>[6x]MLAFPKEFWWGGATSGPQSEGRFAKQHRNLFDYWYEEEPDLFYDYVGPDTASDAYHQIESDLTLLASLGHNSYRTSIQWTRLIDDFEQATINPDGLAYYNRVIDACLANGIRPVINLHHFDLPIALYQAYGGWESKHVVDLFVAFSKVCFEQFGDRVKDWFVHNEPMVVVEGSYLMQFHYPAIVDGKKAVQVAYNLALATAKVIQAYRRGPAELSDGRIGTILNLTPAYPASQSEADMA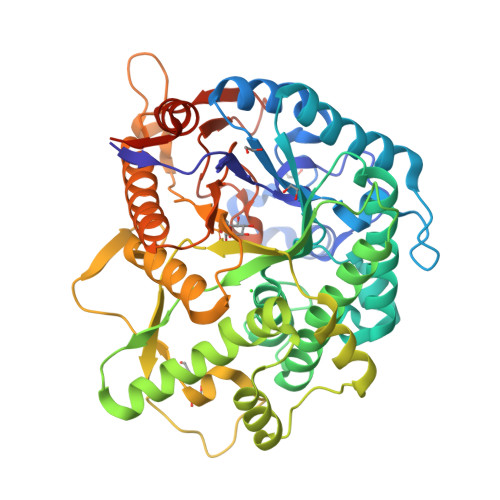AAHFAELWNNDLFMEAAVHGKFPEELVAVLKKDGVLWQSTPEELALIAENRVDYLGLNFYHPKRVKAPDAIPVISPSWSPEWYYDPYLMPGHRMNVDKGWEIYPEAVYDIAIKMRDHYDNIPWFLSENGVGISGEDRYRDETGQIQDDYRIQFLKEHLTYLHKGIEAGSNCFGYHVWTPIDGWSWLNAYKNRYGLVENNIHTQVRRPKASAYWFKKVATHNRLISLEVMEEFGGSASHLSD>[2x]TPYDYIIVGAGPGGIIAADRLSEAGKKVLLLERGGPSTKQTGGTYVAPWATSSGLTKFDIPGLFESLFTDSNPFWWCKDITVFAGCLVGGGTSVNGALYWYPNDGDFSSSVGWPSSWTNHAPYTSKLSSRLPSTDHPSTDGQR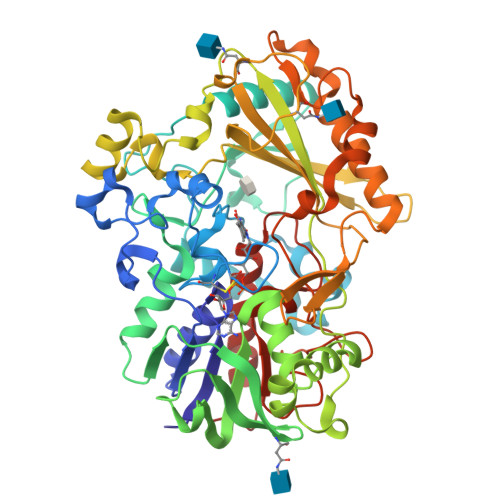YLEQSFNVVSQLLKGQGYNQATINDNPNYKDHVFGYSAFDFLNGKRAGPVATYLQTALARPNFTFKTNVMVSNVVRNGSQILGVQTNDPTLGPNGFIPVTPKGRVILSAGAFGTSRILFQSGIGPTDMIQTVQSNPTAAAALPPQNQWINLPVGMNAQDNPSINLVFTHPSIDAYENWADVWSNPRPADAAQYLANQSGVFAGASPKLNFWRAYSGSDGFTRYAQGTVRPGAASVNSSLPYNASQIFTITVYLSTGIQSRGRIGIDAALRGTVLTPPWLVNPVDKTVLLQALHDVVSNIGSIPGLTMITPDVTQTLEEYVDAYDPATMNSNHWVSSTTIGSSPQSAVVDSNVKVFGTNNLFIVDAGIIPHLPTGNPQGTLMSAAEQAAAKILALAGGP> MLKDLVREKLLTIMNTKAYTQFNPEQLLQLENEMKIYMKSGDSALTEGNYFFLMEMLFYVLVYRNQDVDAQVVYNTLRDRLGENSYKMVIMKATLLQINGNDKGAIEYL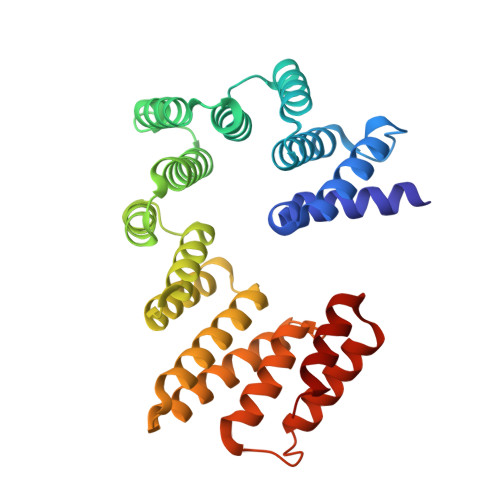ENLLNDDLEYETDFVTYVSIAKKLIAIKTTSKNLSQESVLKEVVALTDKFPLDAELWWYASEIYFEMGQFEKACYCLEQVLCITPFNYACFGRLSETLYYEALRSKKQTKTELLEKALKNALRSVELSELYLKGWALVNIISRELGRNKQNDLIKLSASKLKEISAKSNNKDKITAELILNKI Pantothenate kinase (PANK, EC 2.7.1.33) is the first and rate-controlling step in the only pathway for coenzyme A (CoA) biosynthesis. The isoform expression level and potent feedback inhibition by acyl-CoAs control the intracellular CoA content. Within the cell, the PANK3 dimer exists in one of two distinct conformations: the inactive conformation stabilized by the binding of acetyl-CoA and the active conformation stabilized by the binding of ATP•Mg2+.

The crystal structure of the PANK3•AMPPNP•Mg2+•PZ-2891 complex reveals that PZ-2891 binds across the dimer interface to simultaneously interact with both PANK3 protomers. The ‘ring of ligands’ linking the two protomers explains the high thermal stability of the complex. The isopropyl moiety packs into a hydrophobic cavity created by V250′, I253′, Y254′, Y258′, and A269′ located on the flexible flap that is disordered in the PANK3•AMPPNP•Mg2+ complex9 but becomes structured in the PANK3•AMPPNP•Mg2+•PZ-2891 complex. The carbonyl group forms hydrogen bond interactions with R207, which explains the lack of PZ-3067 binding. The piperazine ring acts as a spacer to present the pyridazine ring to the opposite protomer to hydrogen bond with R306′ and engage W341′ by π-π stacking interactions. PZ-2891 interaction with R306′ also allows an inter-protomer hydrogen bond between R306′ and T209 to further stabilize the dimer. Comparison of the PANK3•AMPPNP•Mg2+•PZ-2891 complex to the PANK3•AMPPNP•Mg2+•pantothenate complex shows that pantothenate and PZ-2891 both form hydrogen bonds with R207, and the isopropyl substituent of PZ-2891 docks into the hydrophobic cavity occupied by the dimethyl group of pantothenate. However, pantothenate does not interact with the dimer interface, and the connection between R306′ and T209 in the pantothenate complex is mediated by a water molecule rather than by a direct hydrogen bond. The structural analysis suggests that PZ-2891 first binds to the pantothenate site of the PANK3•ATP•Mg2+ complex followed by closing of the flexible loop, and the engagement and re-organization of the dimer interface. The induced fit mechanism is the most common binding mode observed in high-affinity inhibitors, and with PZ-2891 the two protomers become locked together to create a structure that is distinct from the structures of all the normal catalytic intermediates.

> MGSSHHHHHHSSGLVPRGSPWFGMDIGGTLVKLSYFEPIDITAEEEQEEVESLKSIRKYLTSNVAYGSTGIRDVHLELKDLTLFGRRGNLHFIRFPTQDLPTFIQMGRDKNFSTLQTVLCATGGGAYKFEKDFRTIGNLHLHKLDELDCLVKGLLYIDSVSFNGQAECYYFANASEPERCQKMPFNLDDPYPLLVVNIGSGVSILAVHSKDNYKRVTGTSLGGGTFLGLCSLLTGCESFEEALEMASKGDSTQADKLVRDIYGGDYERFGLPGWAVASSFGNMIYKEKRESVSKEDLARATLVTITNNIGSVARMCAVNEKINRVVFVGNFLRVNTLSMKLLAYALDYWSKGQLKALFLEHEGYFGAVGALLGLPNFSDD>[6x]MSHLKNILFIIIVSLFFISSCSTVMSTEGWFMPFDNWLYQLQNADPVEISSSGFEIAVIDYSKDGSESGEYSPEEIKIMVDAGVVPVAYV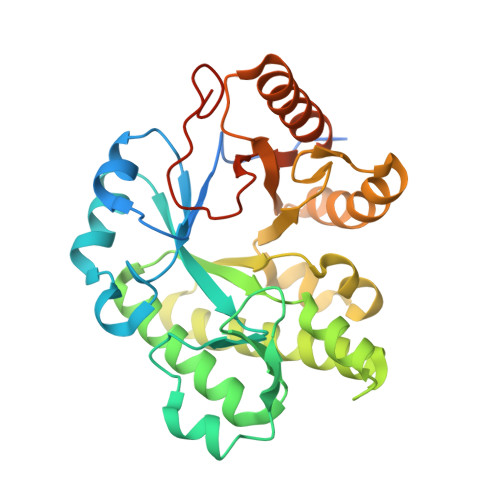NIGQAEDYRFYWKESWYTNTPEWLGEEDPAWPGNYFVKYWYNEWKEIVFSYLDRVIDQGFKGIYLDRIDSFEYWAQEGVISRRSAARKMINFVLEIAEYVRERKPDMLIIPQNGENILDFDDGQLASTVSGWAVENLFYLKTIPLEENETKSRLEYLIRLNRKGKFILSVDYVDDGSDSFENISRILDYYEKAKRNGCIPYAARSDLELDEMNVIEGIQPPEALKDYESRTYR>MQEEAKLTKANNRFGLRLLRALPSGPEKNVFFSPYSVSTAMGMAFAGARGQTQQELSQGLGFSDVDLTDAGVLDAYTHHTERLKSTPSNSTLDVANAAAIQRTLALLNSYESALQSSFGAELHKVDFAGEPQAAVDFVNNWVKRKTHDKIEKLFNEPLDPDTLLVLLNAIYFKGEWNTAFVKEHTEKRQFFNGGVTPVEVDTMRLEARIKYRFFDDLQVEVVELPYRGLDYTMAILLPKENTGVEGLKQNLTIDRFQNYLSDLRERKITVLLPKFKLETKYSLKAPLQSLGIKQIFESGADLSGINDGSLRVSAVEHKAVVEVNEEGTVAAATTGVVIVPYSLGPEPVVFRVDHPFLFFIR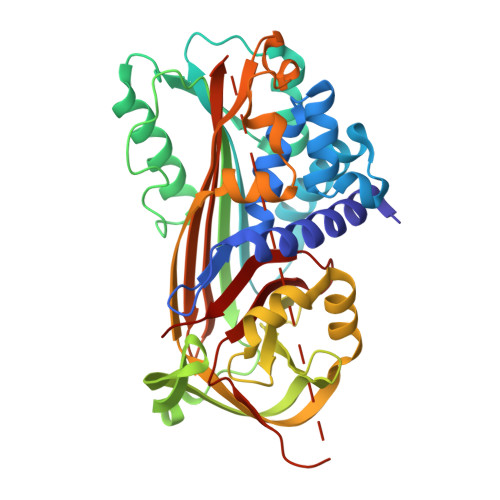NTRTDDIFFVGQVNKL[2x]>[4x]MGMSPRPQIKVGVLGATGTVGQRFIELLAAHPYFALHALGASSRSAGQQYARVVRWKLPSPIPDAVRHMVVHECRPDAPGF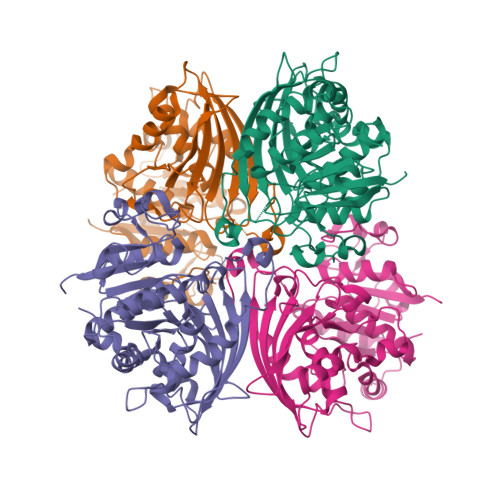AECGVVFSGLDADVAGDIENAFRAADLVVYSNAKNYRRDPLCPLIVPLVNPSHLSIIPYQREQLGLKKGYIVTNANCSTTGIVVPLAALEKAFGPLDTVIVTTLQAISGAGYPGVSSLDIMDNVVPLISGEEDKIEWETNKILGGVTPDNKAFDLHAPKQINVSATCTRVPVIDGHTGCVSVKFARSPPPSVAEVENAFREYTCDAQHLGVPSAPAQAIVVHDAPDRPQPRLDKNLHNGACVSVGRIRECPVFDIKFVCLIDNVRLGAATSSIINAEIAVEKGLIQLEHHHHHH> LPTSNPAQELEARQLGRTTRDDLINGNSASCADVIFIYARGSTETGNLGTLGPSIASNLESAFGKDGVWIQGVGGAYRATLGDNALPRGTSSAAIREMLGLFQQANTKCPDATLIAGGYSQGAALAAASIEDLDSAIRDKIAGTVLFGYTKNLQNRGRIPNYPADRTKVFCNTGDLVCTGSLIVAAPHLA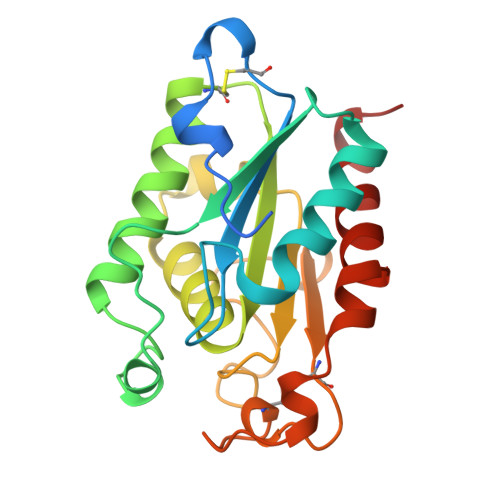YGPDARGPAPEFLIEKVRAVRGSA>WSHPQFEKIEGRMSDGRESFLEVMRSVYERYLVGVPGVSEVWLIAHADSYTGLEDYDGDPRDPALSEKGRAQARLLAARLAGVPLHGVWASGAHRAQQTASAVAAEHGLRVRTDARLREVRTNWDDGRPS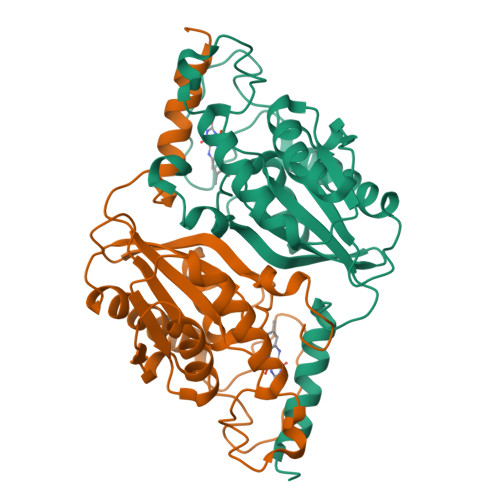ELKPHGVYPFPEPEKEVAERMRTAVTAAVAATPPAPDGTTRVAVVGHDSALVILMGSLMNLGWGQLDMILPLTSVSVLAVKDERMVVRSIGDATHLAAAPSDVI[4x]> SPVAGQKYDYILVGGGTAACVLANRLSADGSKRVLVLEAGPDNTSRDVKIPAAITRLFRSPLDWNLFSELQEQLAERQIYMARGRLLGGSSATNATLYHRGAAGDYDAWGVEGWSSEDVLSWFVQAETNADFGPGAYHGSGGPM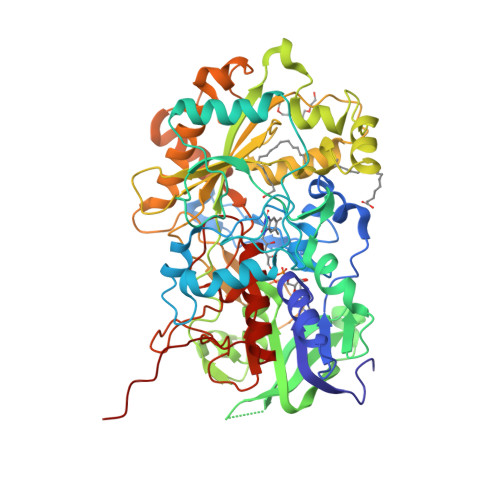RVENPRYTNKQLHTAFFKAAEEVGLTPNSDFNDWSHDHAGYGTFQVMQDKGTRADMYRQYLKPVLGRRNLQVLTGAAVTKVNIDQAAGKAQALGVEFSTDGPTGERLSAELAPGGEVIMCAGAVHTPFLLKHSGVGPSAELKEFGIPVVSNLAGVGQNLQDQPACLTAAPVKEKYDGIAISDHIYNEKGQIRKRAIASYLLGGRGGLTSTGCDRGAFVRTAGQALPDLQVKFVPGMALDPDGVSTYVRFAKFQSQGLKWPSGITMQLIACRPQSTGSVGLKSADPFAPPKLSPGYLTDKDGADLATLRKGIHWARDVARSSALSEYLDGELFPGSGVVSDDQIDEYIRRSIHSSNAITGTCKMGNAGDSSSVVDNQLRVHGVEGLRVVDASVVPKIPGGQTGAPVVMIAERAAALLTGKATIGASAAAPATVAA>MNNEIGRKITSLTLMTIMVAGGLTFAIPGVMPEAMAANANLFVSAENSQFDNYMSGPQVIEVVVIDSDINDTDEAKGEPDVTVNGKVLRMVQAVDGNWYGYFADRDQAQIADSTATTADSGLDFGVFCASSSGTAALGFSTTETDGIAIPITIANATATGNGTQTGSSSGGAITTTCAANTLDASTANGTINVVREAKDPVAASGSVSVGQIGLKNGTANSGPNWPFIQLYELNPTGNVVVQYNKGGGVQSTTLTFDTVDQFAELSLDRTVFPRVSQVHATITDLWLNIDPTDEDSWTFATNTKNTTSSFNVDTFYQVFDENGASGGSALTLRTTLSSLMCEDNCVLTLDVDAQSSGTPVVTIQDNGDSILTQLNASSNTNANNASAFGISTETAKLGTGSIPVTITEQGPNSGVFGTYDESDKSVLKITDNAKRGTSASLDYNETPQTILVGFSFASIDIQPVTDEWTSGQEIPVVIVDADQNKNSRADEDLDLNNPDVTLIPALRTGDPFTIDEGGTPSLIFTNGTNGDDSIFDTGAINNTSAGQVGNFTLNIN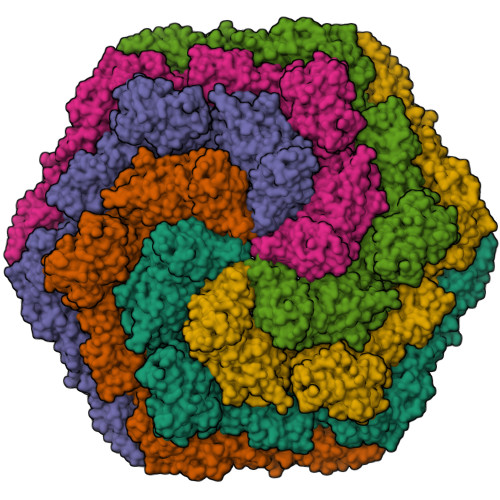VTRFSSATNITSTESIDTFSKRLISAQTANSSANFDVDFAIIDLGSATLETLKETVVDEDNTAVGFNFFNYDVRSLGADTVSIALLNTTGNILPWVNNDTRNVDKNNAILLVSNSTNSQAYVDLTNAVSDAVYGSTNTDSNVNIGFAMYFTGVGDLAAKEVIVMDFFSFGFTDDGVQSSERFANQIIRIEAEETGDNTSTFEGSLEYVMVNQINIQDAGTFSGITPIADDPSFIVIEDLTDEDAPRVNYNDLGADGVTTPVSDQEEAPSHSGVVSLNADSYKIADTVVITVEDLDLNVDSDLIDIFTVVSDNSKATDDAVGSATTQSLSFGELGRLLDVTFDDVIWSTPDGANNTATGNDSDTCSTELSNAGITDTGLGATGFTLVETGAATGVFVGDFQIPSFWCRVSDTTTTPYTYAGDEETTTGLDIEVNYVDFRDASGEIVEVGDSAGVRANTGSVSLDRTVYPVPFGTIADSSKAANAAPNGRSVFPIHATGITSTIDSTEELPTGDLTIHVRINDPDFDENPAGEDAMDQDNALKISVIRGSDSVVLGYAGASERTGKIDVGGNNGTISNIRSFGEMDEIAPDAGIFELDVNIKFTDGPASAQCNSHDTLYTALDGTTGKADTNRFDDGAASGQEYCILQGDILQVEYTDPADASGDANTVTDSATFDLRNGVLQSDKSVYIIGSDMILTLIEPDFDLDNDSAETYDLDLIEWDSDAATTTMGNKGVTGAAAAFDPEPTDFRETGDSTGIFQIVIEIPESLSNDKLERGEEIILEYTDWGPSGSDYVGDEDEDVNLTIYTSNFGATVELDQKVYSWTDKVYITIVAPDHNFDSDLVDEIGETDSDPIKVSTRGFDLDNYKLVETGTDTGIFTGEVILTGFTAHDADGDGNTGDATGTTSGSGPTDGLLATDDDDGLTVSFEFSEDETIVGSALIRWNIGEVQWLEASYPASGTGVVRVIDPDMNLDPEAVDNFEVDVWSDSDAGGIDLTVTETNEATGIFEGTVFFTTLDESSGHRLRVSEGDTVTAEYEDNTLPDPYTTADELDITATSLIGTVVPPLERAPAANLRTVDAFGNSLDSVSVDQQVQISADLANGQDREQSFAYLVQIQDANGVTVSLAWITGSLSSGQSFSPALSWIPTEAGTYTATAFVWESVDNPTALSPPVSTTVNVS[6x]> DLSRSDEIQKARIQLPVFGEEHKIMEAIHHNDVVIICGETGSGKTTQVPQFLYEAGFGAEDSPDYPGMVGITQPRRVAAVSMAERVANELGDHGHKVGYQIRFDSTAKEDTKVKFMTDGVLLREMMHD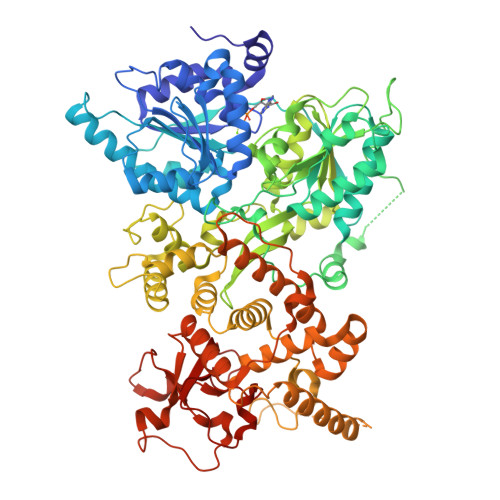FKLTKYSSIIIDEAHERNINTDILIGMLSRCVRLRAKLHKENPIEHKKLKLIIMSATLRVSDFSENKTLFPIAPPVLQVDARQFPVSIHFNRRTAFNYTDEAFRKTCKIHQKLPPGAILVFLTGQQEITHMVKRLRKEFPFKKNSKYNKDLETPVSKMGINSKTTDLEAEDIDFSVQVIDQDKFKSAIRYEEDEGNSGNGEDEEDEEEEGFEEVLTEGQTANDPLYVLPLYSLLPTKEQMRVFQKPPQGSRLCIVATNVAETSLTIPGVRYVVDSGRSKERKYNESNGVQSFEVGWVSKASANQRSGRAGRTGPGHCYRLYSSAVFEHDFEQFSKPEILRMPVESIVLQMKSMAIHNIINFPFPTPPDRVALSKAIQLLQYLGALDNKEMITEDGKKMSLFPLSPRFSKMLLVSDEKACLPYIVAIVSALSVGDPFINEFELGINEISRKPNPDENLDDKIREHDESTPGMDPELKKELRSKFYKSRSQFSKLDKFSDVFRLLSVVSAMDYVPKEQKEIFMKKNFLRGKLMEEIVKLRKQLMYIIKSNTSKENIAVVIRNEDLKSDIPSVIQIKLLKQMICAGFVDHVAVRADVLFPDDAKITNRTSIINIPYIPVLATRTPNIEDCFVYIHPTSILNNLGEMPPKYMLYYSLHLGGNNKTRMNTLCDIA>AMRIVFDIGGSVLVPENPDIDFIKEIAYQLTKVSEDHEVAVVVGGGKLARKYIEVAEKFNSSETFKDFIGIQITRANAMLLIAALREKAYPVVVEDFWEAWKAVQLKKIPVMGGTHPGHTTDAVAALLAEFLKADLLVVITNVDGVYTADPKKDPTAKKIKKMKPEELLEIVGKGIEKAGSSSVIDPLAAKIIARSGIKT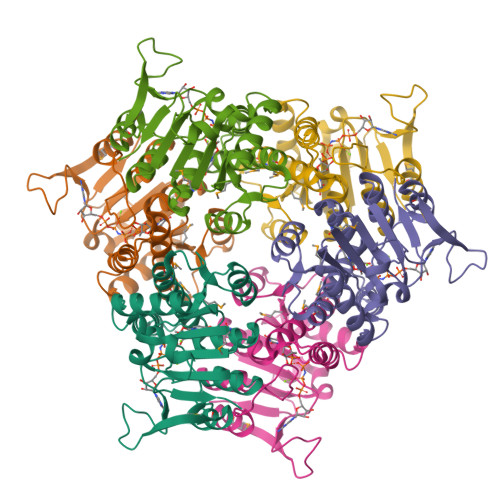IVIGKEDAKDLFRVIKGDHNGTTIEP[2x]Aspartate aminotransferase (AspAT) catalyzes the reaction from L-glutamate and oxaloacetate to L-aspartate and α-ketoglutarate. AspAT utilizes pyridoxal 5’-phosphate (PLP, Vitamin B6) as a cofactor and is the most extensively studied PLP-dependent enzyme. Among the five classes, AspAT proteins belong to class I AT that is further divided into 2 subcategories, subgroup Ia and Ib. In this study, we report a crystal structure of AspAT from Corynebacterium glutamicum ATCC13032 (CgAspAT) in complex with a PLP and citrate molecule.

In order to elucidate the molecular mechanism of CgAspAT, we determined the crystal structure of the protein at 2.0 Å. There were two CgAspAT molecules in each asymmetric unit, which form a homodimer of the protein. Dimerization is mainly mediated through the contact between the core domains of the two subunits with three α-helices (α6, α8, and α12) of one molecule in contact with the corresponding α-helices of the other molecule. Since we observed the electron density for the PLP cofactor in our structure without adding it in the crystallization process, we speculate that the PLP cofactor binds strongly to CgAspAT. Unlike the binding of the phosphate moiety in other AspAT enzymes, where side chains of arginine, threonine, and one or two serine residues are involved, the moiety of CgAspAT was stabilized by the side chains of one tyrosine (Tyr73) and four serine residues (Ser103, Ser104, Ser256, and Ser258) through a hydrogen bond network. Near the aldehyde group of the bound PLP, we observed the conserved Lys259 residue. Because the citrate molecule is stabilized by hydrogen bonds with the highly positively-charged residues such as Arg39, Lys41, Arg144 and Arg394, binding of the citrate molecule seems to mimic the substrate binding of CgAspAT. When we replace the Arg39, Tyr142, Arg144, Asn191 and Arg394 residues by alanine, all mutants showed reduced or almost complete loss of enzyme activity, indicating that these unique residues are crucial for the binding of the glutamate substrate in CgAspAT. However, in CgAspAT, the N-terminal region is positioned away from the core domain and is not involved in the formation of the substrate binding-site. However, CgAspAT shows only 10~15% amino acid sequence similarity with AspATs from subgroup Ia and subgroup Ib and exhibits unique structural features not only in the auxiliary domain but also at the catalytic and substrate binding sites. These amino acid sequence analysis and the structural comparisons reveal that CgAspAT does not belong to either subgroup Ia or subgroup Ib, but rather should be classified to a new category, subgroup Ic.

>MSSVSLQDFDAERIGLFHEDIKRKFDELKSKNLKLDLTRGKPSSEQLDFADELLALPGKGDFKAADGTDVRNYGGLDGIVDIRQIWADLLGVPVEQVLAGDASSLNIMFDVISWSYIFGNNDSVQPWSKEETVKWICPVPGYDRHFSITERFGFEMISVPMNEDGPDMDAVEELVKNPQVKGMWVVPVFSNPTGFTVTEDVAKRLSAMETAAPDFRVVWDNAYAVHTLTDEFPEVIDIVGLGEAAGNPNRFWAFTSTSKITLAGAGVSFFLTSAENRKWYTGHAGIRGIGPNKVNQLAHARYFGDAEGVRAVMRKHAASLAPKFNKVLEILDSRLAEYGVAQWTVPAGGYFISLDVVPGTASRVAELAKEAGIALTGAGSSYPLRQDPENKNLRLAPSLPPVEELEVAMDGVATCVLLAAAEHYANLEHHHHHH[2x]> MIEKLIHFINNDLLEGAADDLDQNTPLLELGILDS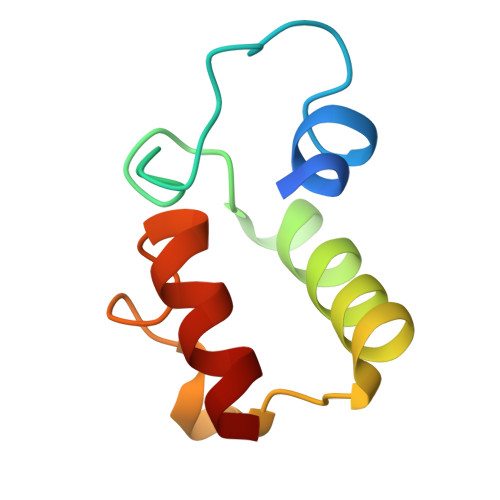LSMVLLLAHIDQQYGVKIPEHEINPEHFENVATLAALINQLS> GPDSSQCESPSLTEL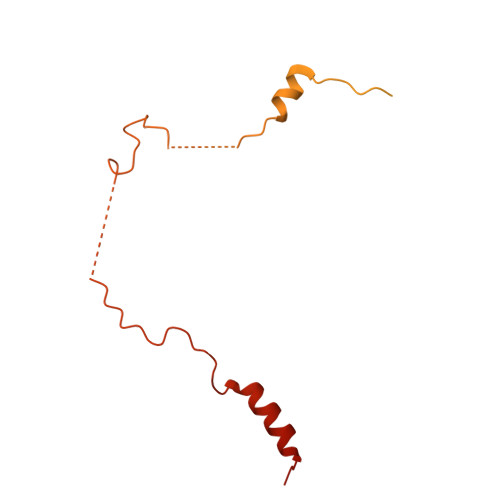FQEHKENNISQCFTLSDLCNQSSASFTDLSLGSFPLSQLANRCQSSPGISELTGSLSSLAFHKASPTRDLENLSLSELIAETIDVDNSQIKKESFEVSLSEVRSPGIDSNIDLSVLIKNPDFVPKPVVDPSIAPSSRTKVLSSKLGKNSNFAKDNKKNNKGSLTRKPPFSLSWTKALAARPSAFASTLCLRYPLKSCKRRTLDLYKTFLYSRQVQDVKDKEISPLVAITPFDFKSASPDDIVKANQKKAFTRELEVLFQ> FNQTQPERGDNNLTRIVGGQECKDGEC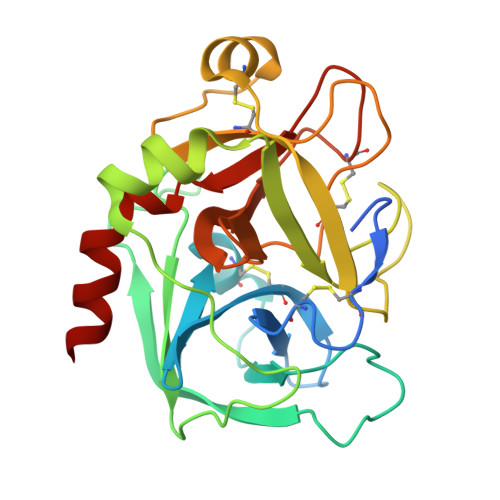PWQALLINEENEGFCGGTILSEFYILTAAHCLYQAKRFKVRVGDRNTEQEEGGEAVHEVEVVIKHNRFTKETYDFDIAVLRLKTPITFRMNVAPACLPERDWAESTLMTQKTGIVSGFGRTHEKGRQSTRLKMLEVPYVDRNSCKLSSSFIITQNMFCAGYDTKQEDACQGDSGGPHVTRFKDTYFVTGIVSWGEGCARKGKYGIYTKVTAFLKWIDRSMKT> QAEEWYFGKITRRESERLLLNPENPRGTFLVRESETTKGAYCLS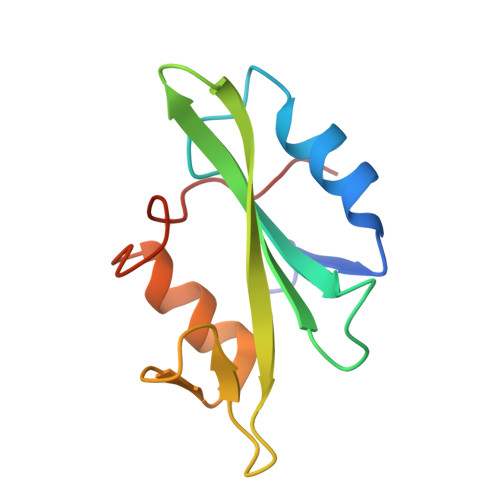VSDFDNAKGLNVKHYKIRKLDSGGFYITSRTQFSSLQQLVAYYSKHADGLCHRLTNVCPT(2S)-2-{[(S)-[(1R)-1-aminoethyl](hydroxy)phosphoryl]methyl}butanedioic acid | C7 H14 N O6 P | 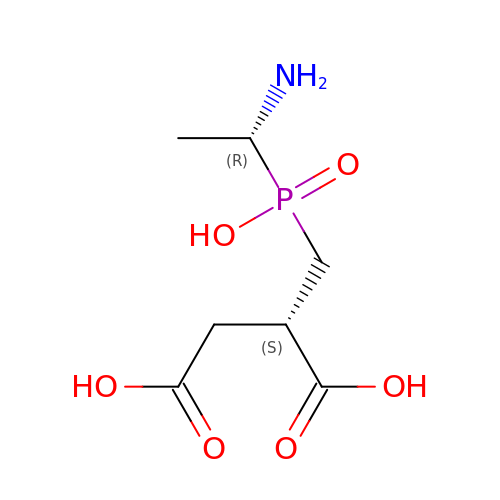LWODXTSWCZWQHR-RFZPGFLSSA-N N,N-BIS(3-D-GLUCONAMIDOPROPYL)DEOXYCHOLAMIDE | C42 H75 N3 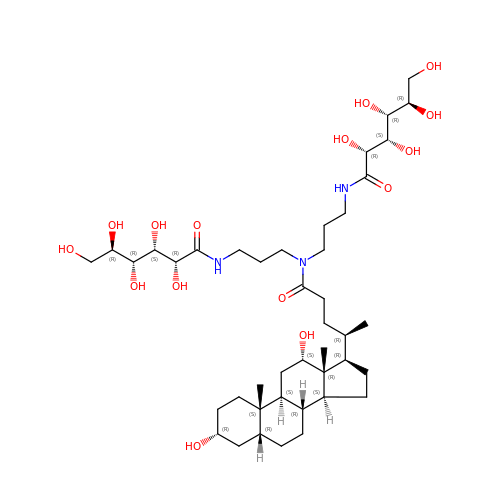O15 | OJSUWTDDXLCUFR-HGZMBBKESA-N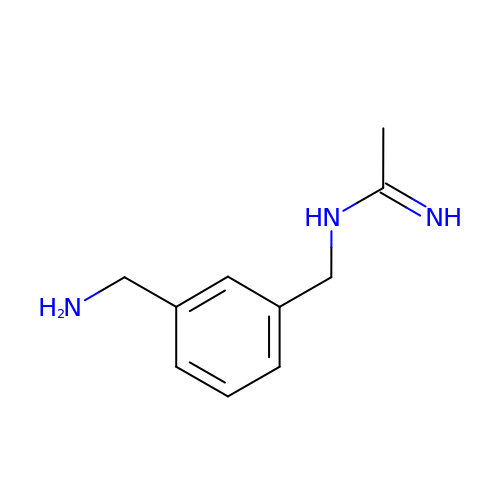N-(3-(AMINOMETHYL)BENZYL)ACETAMIDINE | C10 H15 N3 | RODUKNYOEVZQPR-UHFFFAOYSA-N We characterized CtGH76 from the sordariomycete Chaetomium thermophilum, a member of the Fungi/Bacteria-mixed GH76 subfamily, revealing conserved structural features and functional divergence within the GH76 family. Notably, our structural characterization by X-ray crystallography combined with glycan fragment screening indicated that CtGH76 can recognize GPI-anchors like members of the Dfg5 subfamily but shows a broader promiscuity toward other glycans with central α1,6-mannobiose motifs due to the presence of an elongated glycan-binding canyon. Here, we present the crystal structure of a novel fungal GH76 member from the F/B-mixed subfamily, in complexes with different glycans and glycan fragments. Together with structural bioinformatics, we found that members of the F/B-mixed subfamily act as secreted GHs in glycan degradation, which includes not only α1,6-mannans but also GPI-core glycans. Compared to other GH76 orthologs, our findings demonstrate that CtGH76 features an elongated glycan-binding canyon, adept at accommodating a wider range of complex glycans.

To exclude the residual α1,6-mannasidase activity of CtGH76 under crystal soaking conditions, we generated single-site mutants for its catalytic DD motif. For the active-site mutants D164N and D163N, soaking with α1,6-mannotriose resulted in α1,6-mannobiose binding to subsites −1/−2, alongside with single mannose residues at subsites +3 and −4. When comparing the wild-type of CtGH76 with its aspartate mutants after soaking with α1,6-mannotriose, sugar residues at subsites −4, −2, and +3 adopt nearly identical conformations. However, occupancy of subsite −1 is observed only in the active-site mutants, with slight variations in orientation. Glycan mapping revealed that the putative substrate binding site of wild-type CtGH76 contains only single mannose units for α1,6-mannotriose, whereas DD motif mutants accommodate both mannose and α1,6-mannobiose within the binding canyon. Reduced activities of DD motif mutants, as observed in corresponding S. cerevisiae Dfg5 mutants, result in a complete loss of function.

> MAGIADLTAALASADRNRVTRVEAMRRSPTTISLSTLGALSALWGILYFMTCSGRNSRGVLADASSGMLQTRQSDSESLNSTGLAQAAINGLNARFYESSNARWSSDEPWWISGVALTMVIEYMRRSGSKEYLDQVEDVIEVQRQPLSWWPSGEGEFRADATNDTGWWALAMVRMYDLTGNEDYLNISIKDEAYMRQWWTDTECGGGLYVDIQDLTYKNAIANELYLKLVASLANRAPNATIYLDRAQQAWTWFLGSGMINGVNLINDGLARDSNTGSCYNNRLPVWTYNQGVILGALVELYHATKDESYLLSAQAIADAVLSPSNGLTSSSGVLTETCEGSDSCNQDQQVFKGVFALNLAELGDAVAGASSDPDAGQDYREYLDTNMQSMYANDRSEIVPTLFDSSTGDLYDVSWSGPFRNATMPKQASAIGLYVANI>MEIKETYDFSSIVDLWNKNIGTVYPMNLELFKQNYINDRQRKKIMGAFNGEILIGFVIYKQWTYKSGSLKPNHKIGYINSIIVDINFRHQGIGTKLLDAAEEELINSGVKILRCGSDTYHFFPGIPLECLPSEEFFLVRGYKMQDYFYDLIGDVSKVDFKKPSIKDGFKVNVMKPEDRKGLFEFLEKSFSGRWLEEFIEFFQVGMKERDIVLIKYKTSVIGFSHIYDNKSSFIGPPIYWKALLGHNYGGLGPIGIDKTYRKQGLGRLLLYESLQILKKR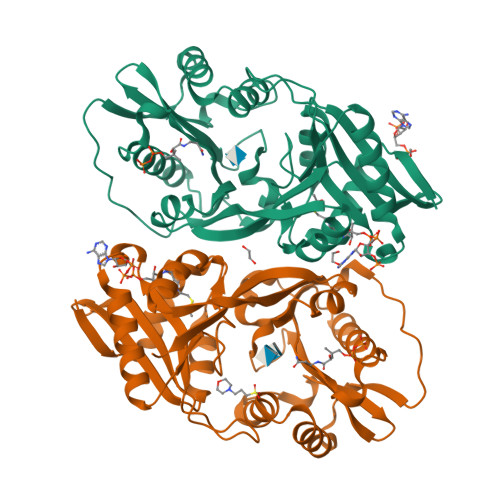EVKKMVIDWTEKDIINFYGRFNFMPWKAYRKATKEVKDGKGGGHHHHHH[2x]> STITDEDELTGILKKLSLEKYQPIFEEQ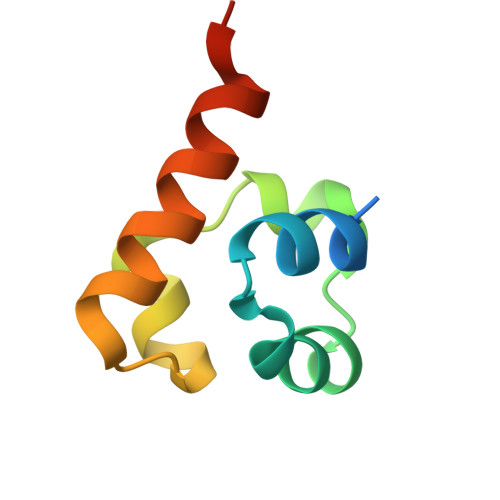EVDMEAFLTLTDGDLKELGIKTDGSRQQILAAISELNAGKGRE>SNAMQKSVLEQLKQVTMVVADTGDFELIKKYKPVDATTNPSLILKAVKEQKYSNLVAETISKVKANNPDLNSDDLVKEIAIEILVSFGIKILDVIEGKVSSEVDARVSFNSATTIDYAKRIIARYESNGIPKDRVLIKIAATWEGIKAAKLLQKEGINCNLTLIFDKAQAKACAEAGVYLVSPFVGRITDWQMQQNNLKTFPAIADDDGVNSVKAIYKLYKSHGFKTIVMGASFRNVEQVIALA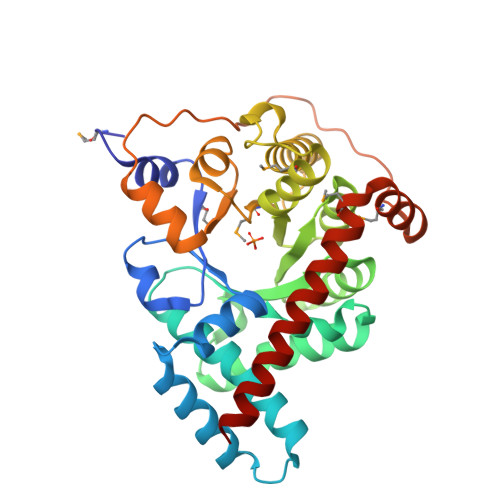GCDALTISPVLLEELKNRDEHLEVKLTKNDDVVTQSPQISEADFRWLMNENAMATHKLAEGIRLFTKDTIELENIIKQNL[2x]> MQYSIEKLKKEENSLAKDYYIYRLLEKNKISKKDAQDLQSHIFRYIGKIKSELEKIIPLKPYINPKYAKCYTYTANTILDANLTCQSVRLNSLVFIASLNSKDRTTLAQTFKNQRPDLTNLLLAFNTSDPMSYIVQKEDINGFFKLYNYSKKYDLDLNTSLVNKLPNHIGFKDFAQNIIIKKENPKFRHSMLEINPENVSEDSAFYLGVNALTYDKTELAYDFFKKAAQSFKSQSNKDNAIFWMWLIKNNEEDLKTLSQSSSLNIYSLYAKELTNTPFPKIESLNPSKKKNNFNMQDPFAWQKINKQIRDANASQLDVLAKEFDTQETLPIYAYILERKNNFKKHYFIMPYYDNIKDYNKTRQALILAIARQESRFIPTAISVSYALGMMQFMPFLANHIGEKELKIPNFDQDFMFKPEIAYYFGNYHLNYLESRLKSPLFVAYAYNGGIGFTNRMLARNDMFKTGKFEPFLSMELVPYQESRIYGKKVLANYIVYRHLLNDSIKISDIFENLIQNKANDLNKS

We report here structure-function studies of soluble periplasmic LT of Campylobacter jejuni. The LT Cj0843 was identified from a virulent strain of C. jejuni and localized in the periplasm. The LT enzymes cleave the PG MurNAc-GlcNAc glycosidic bond similar to lysozyme with the noted difference that LTs have an additional (2nd) cyclization step; this step requires a boat conformation of MurNAc leading to a 1,6-anhydromuramyl product as the predominant terminal saccharide moiety. The crystal structure of the soluble LT Cj0843 from C. jejuni revealed an unusual doughnut-shaped structure containing four domains: NU-, U-, L-, and C-domains.

The structures from both crystal forms are very similar with a root-mean-square-deviation (RMSD) for 509 Cα atoms of 0.75 Å. At the N-terminus is a small helical domain (NU-domain) connected via a flexible linker to the helical U-domain. This flexible linker (residues 75–83) is partially resolved in the P3121 crystal form and fully resolved in the I23 crystal form; it spans 22Å between ordered anchor points I74 and Y84 in the NU-domain and U-domain, respectively. The central pore of the ‘doughnut’ is elliptical and has an inner diameter ranging from 16 to 37Å. The most prominent feature of the electrostatic potential surface of Cj0843 is its predominantly positively charged inner ring surface. The outer ring surface of these ring-shaped proteins shows a more random distribution of positive, negative, and neutral residues. This ensemble of positive charges on the inside of the ring of Cj0843 explains why the majority of sulfate and acetate ions, that co-crystallized at 200mM concentration in both crystal forms, were observed along the inner ring of the doughnut-shaped Cj0843 protein.> MKNVAAAERQLRELESTFDGRLGFVALDTATGARIAHRGDERFPFCSTSKMMLCAAVLARSAGEPALLQRRIAYAKGDLIRYSPITEQHVGAGMSVAELCAATLQYSDNTAANLLIALLGGPQTVTAYARSIGDATFRLDRREPELNTALPGDERDTTTPAAMAASVHRLLVGDALGAAQRAQLNAWMLGNKTGDARIRAGVPADWRVADKTG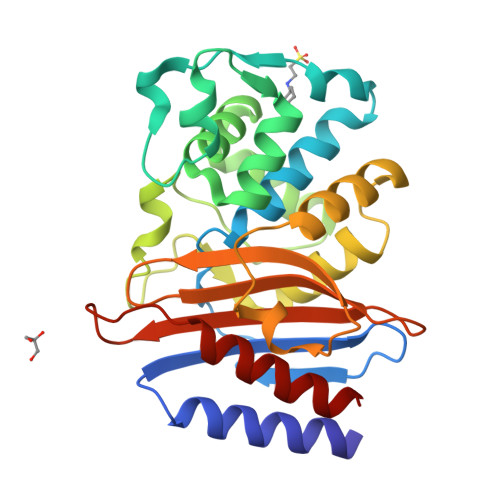TGDYGTANDIGVAYPPNRAPIVFIVYTTMRNPNAQARDDVIASATRIAARAFA>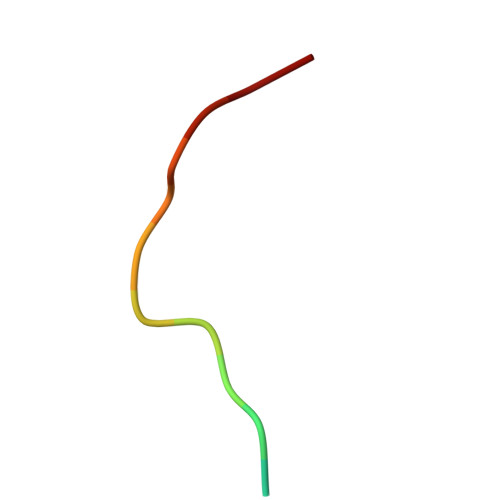 EGSPYVPVHLDASV>[3x]HSVAVIGAPFSQGQKRKGVEHGPAAIREAGLMKRLSSLGCHLKDFGDLSFTPVPKDDLYNNLIVNPRSVGLANQELAEVVSRAVSDGYSCV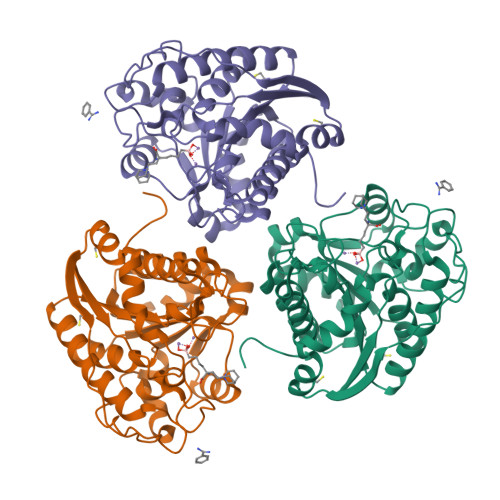TLGGDHSLAIGTISGHARHCPDLCVVWVDAHADINTPLTTSSGNLHGQPVSFLLRELQDKVPQLPGFSWIKPCISSASIVYIGLRDVDPPEHFILKNYDIQYFSMRDIDRLGIQKVMERTFDLLIGKRQRPIHLSFDIDAFDPTLAPATGTPVVGGLTYREGMYIAEEIHNTGLLSALDLVEVNPQLATSEEEAKTTANLAVDVIASSFGQTREG> AGSEQLKCCSGILKEMFAK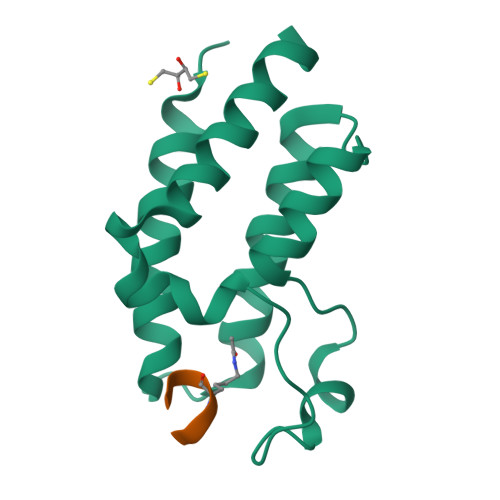KHAAYAWPFYKPVDVEALGLHDYCDIIKHPMDMSTIKSKLEAREYRDAQEFGADVRLMFSNCYKYNPPDHEVVAMARKLQDVFEMRFAKMPD;> TFKSIMK The Drosophila melanogaster centrosome associated protein at 190 kDa (CP190) was first identified as a MAP using MT affinity chromatography. CP190 is a large multi-domain protein that has a distinct localization pattern that is tightly coordinated with the cell cycle. During interphase it is restricted to the nucleus where it serves as a key component of chromatin insulator complexes that spatially organize the genome. Upon nuclear envelope breakdown, a population of CP190 redistributes to the centrosomes and the spindle.

To gain structural insight into the conserved CP190 BTB domain, we purified and crystallized native and selenometionine-substituted BTB (residues 1–135). Crystals belong to the space group P3221 and contain one CP190 BTB molecule in the asymmetric unit. The structure was built and refined to 2.5 Å resolution, yielding R and Rfree values of 21.9 and 25.9, respectively. The final model contains residues 2–121. The BTB domain forms a homodimer across a crystallographic 2-fold axis, adopting a canonical homodimeric structure as found in the BTB-ZF subfamily of BTB domains. Each chain in the homodimer has an α-helical core composed of six helices, α1- α6, flanked by a four stranded β-sheet (β3-β2-β5-β4) and a two-stranded inter-molecular β-sheet formed by β6 and β1' from the homodimeric mate. Key dimer contacts are made at this hydrophobic interface as well as a reciprocal N-terminal β-strand exchange in which β1 extends along the base of the homodimeric mate, forming a two-stranded antiparallel β-sheet with β6'. Along the homodimer’s two-fold axis, α1 makes key hydrophobic interactions with α1' from the homodimeric mate. We analyzed the oligomeric state of the BTB domain using SEC-MALS. We conclude the highly conserved L20 residue is critical to support homodimerization.

> GSHMGEVKSVKVDNWGVFFLQKLQNFFNKTDYCDLTLQFRDNSQLKVHRLVLSACTDYFNVLEQTCEIVDDALIMPNEFQADVVVPIVNFMYTGTLEFELKMYGKLLRTAKEMNMTVLLKLLEAHRRTMENVNRQQRP> MLFQDFTHLYPLSKTVRFELKPIGKTLEHIHAKNFLNQDETMADMYQKVKAILDDYHRDFIADMMGEVKLTKLAEFYDVYLKFRKNPKDDGLQKQLKDLQAVLRKEIVKPIGNGGKYKAGYDRLFGAKLFKDGKELGDLAKFVIAQEGESSPKLAHLAHFEKFSTYFTGFHDNRKNMYSDEDKHTAIAYRLIHENLPRFIDNLQILATIKQKHSALYDQIINELTASGLDVSLASHLDGYHKLLTQEGITAYNTLLGGISGEAGSRKIQGINELINSHHNQHCHKSERIAKLRPLHKQILSDGMGVSFLPSKFADDSEVCQAVNEFYRHYADVFAKVQSLFDGFDDYQKDGIYVEYKNLNELSKQAFGDFALLGRVLDGYYVDVVNPEFNERFAKAKTDNAKAKLTKEKDKFIKGVHSLASLEQAIEHYTARHDDESVQAGKLGQYFKHGLAGVDNPIQKIHNNHSTIKGFLERERPAGERALPKIKSDKSPEIRQLKELLDNALNVAHFAKLLTTKTTLHNQDGNFYGEFGALYDELAKIATLYNKVRDYLSQKPFSTEKYKLNFGNPTLLNGWDLNKEKDNFGVILQ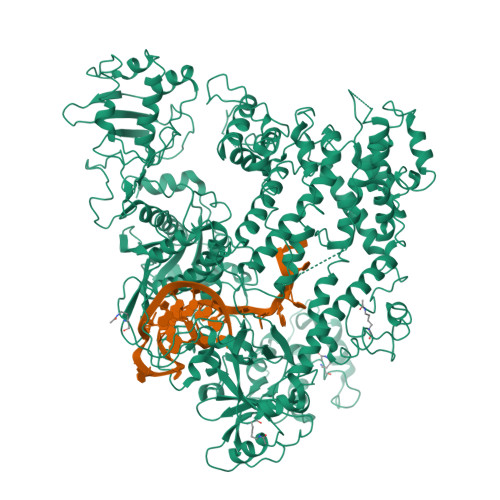KDGCYYLALLDKAHKKVFDNAPNTGKSVYQKMIYKLLPGPNKMLPKVFFAKSNLDYYNPSAELLDKYAQGTHKKGDNFNLKDCHALIDFFKAGINKHPEWQHFGFKFSPTSSYQDLSDFYREVEPQGYQVKFVDINADYINELVEQGQLYLFQIYNKDFSPKAHGKPNLHTLYFKALFSEDNLVNPIYKLNGEAEIFYRKASLDMNETTIHRAGEVLENKNPDNPKKRQFVYDIIKDKRYTQDKFMLHVPITMNFGVQGMTIKEFNKKVNQSIQQYDEVNVIGIDRGERHLLYLTVINSKGEILEQRSLNDITTASANGTQMTTPYHKILDKREIERLNARVGWGEIETIKELKSGYLSHVVHQISQLMLKYNAIVVLEDLNFGFKRGCFKVEKQIYQNFENALIKKLNHLVLKDKADDEIGSYKNALQLTNNFTDLKSIGKQTGFLFYVPAWNTSKIDPETGFVDLLKPRYENIAQSQAFFGKFDKICYNADRGYFEFHIDYAKFNDKAKNSRQIWKICSHGDKRYVYDKTANQNKGATIGVNVNDELKSLFTRYHINDKQPNLVMDICQNNDKEFHKSLMYLLKTLLALRYSNASSDEDFILSPVANDEGVFFNSALADDTQPQNADANGAYHIALKGLWLLNELKNSDDLNKVKLAIDNQTWLNFAQNR> MTIFNLYIFDKFGTLLHYAEWNRTKKSGITREEEAKLTYGMLFSIKSF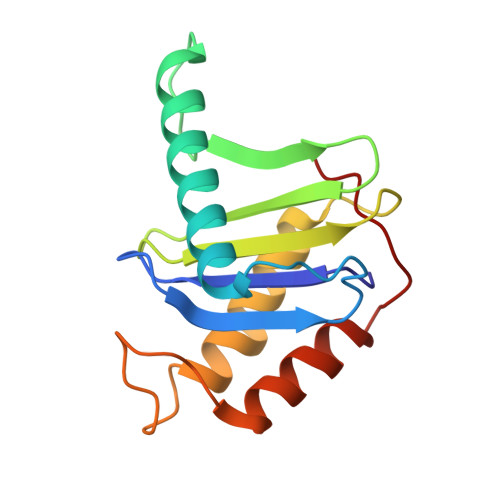VSKISPHDPKEGFLYYKTNRYALHYLETPSGLKFVLNTDTTAINVKELLQQLYAKVWVEFVVRDPLWTPGTVVTSELFQSKLDEFVRQSPIFGIRNI> SEFMEQNPQSQLKLLVTRGKEQGYLTYAEVNDHLPEDIVDSDQIEDIIQMINDMGIQVMEEAPDADDLMLAENTADEDAAEAAAQVLSSVESEIGRTTDPVRMYMREMGTVELLTREGEIDIAKRIEDGINQVQCSVAEYPEAITYLLEQYDRVEAEEARLSDLITGFVDPNAEEDLAPTATHVGSELSQEDLDDDEDEDEEDGDDDSADDDNSIDPELAREKFAELRAQYVVTRDTIKAKGRSHATAQEEILKLSEVFKQFRLVPKQFDYLVNSMRVMMDRVRTQERLIMKLCVEQCKMPKKNFITLFTGNETSDTWFNAAIAMNKPWSEKLHDVSEEVHRALQKLQQIEEETGLTIEQVKDINRRMSIGEAKA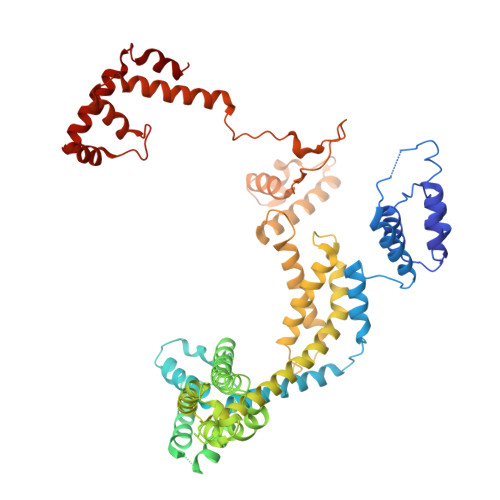RRAKKEMVEANLRLVISIAKKYTNRGLQFLDLIQEGNIGLMKAVDKFEYRRGYKFSTYATWWIRQAITRSIADQARTIRIPVHMIETINKLNRISRQMLQEMGREPTPEELAERMLMPEDKIRKVLKIAKEPISMETPIGDDEDSHLGDFIEDTTLELPLDSATTESLRAATHDVLAGLTAREAKVLRMRFGIDMNTDYTLEEVGKQFDVTRERIRQIEAKALRKLRHPSRSEVLRSFLDD> GAGCAGACCTG;> ACTGCACTCA;> CAAGT;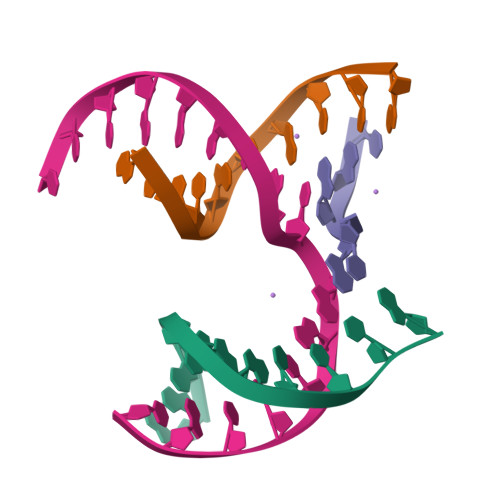> TCTGAGTGCGGTCTGC> SNAAQAETRIGVTIYKYDDNFMSVVRKAIEKDAKASPEITLLMNDSQNDQSKQNDQIDVLLAKGVKALAINLVDPAAAPVVIDKARSNDIPIVFYNKEPSRKALDSYDKAYYVGTDSKESGVIQGELIAKHWQANPEWDLNKDGKIQFVLLKGEPGHPDAEARTTYVIKTLNEKGLPTQQLQLDTAMWDTAQAKDKMDAWLSGPNANKIEVVIANNDAMAMGAVEA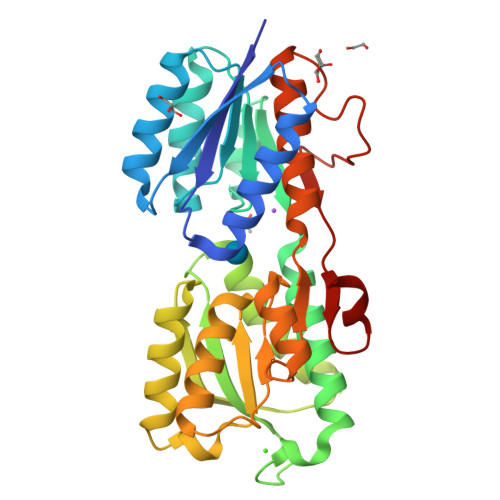LKAHNKTSVPVFGVDALPEALALVKSGQMAGTVLNDANNQAKATFDLAKNLAAGKPAAEGTTWKIENKIVRIPYVGVDKDNLAEFTK> SNAMGAMHVLTLDLAPVTPKDAPLLHRVFHLSPSYFALIGMELPTLEDVVRDLQTLEVDPRRRAFLLFLGQEPVGYLDAKLGYPEAEDATLSLLLIREDHQGRGLGRQALERFAAGLDGVRR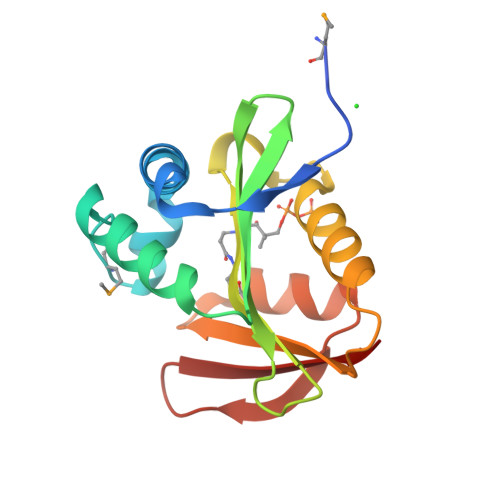LYAVVYGHNPKAKAFFQAQGFRYVKDGGPTLTWYVRPL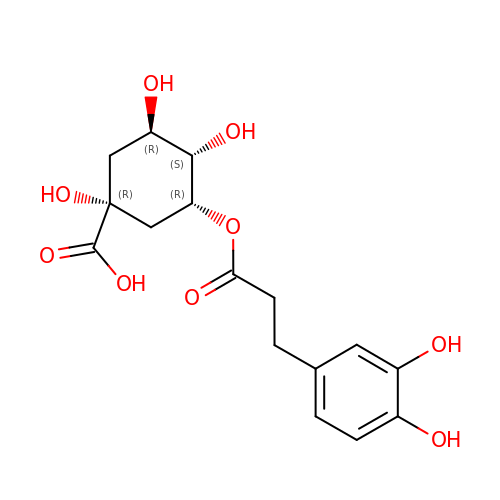(1R,3R,4S,5R)-3-[3-[3,4-bis(oxidanyl)phenyl]propanoyloxy]-1,4,5-tris(oxidanyl)cyclohexane-1-carboxylic acid | C16 H20 O9 | RLGFSACCIOSKQS-UNIGVISCSA-N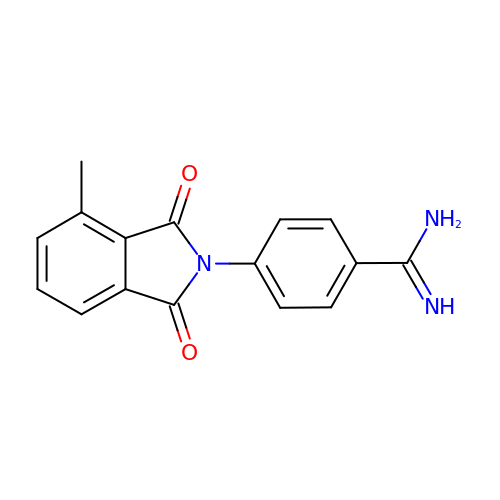4-(4-methyl-1,3-dioxo-1,3-dihydro-2H-isoindol-2-yl)benzenecarboximidamide | C16 H13 N3 O2 | KDWKLFURLBISCV-UHFFFAOYSA-N>MKYMITSKGDEKSDLLRLNMIAGFGEYDMEYDDVEPEIVISIGGDGTFLS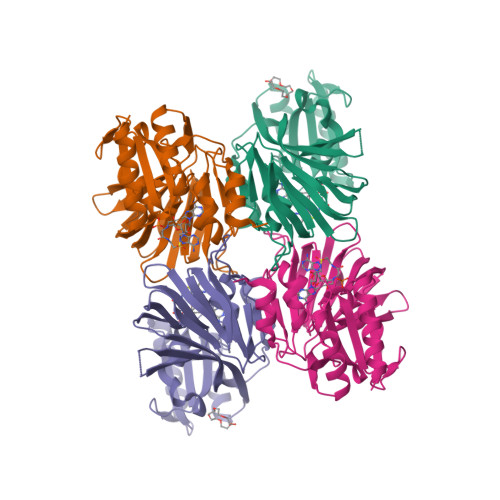AFHQYEERLDEIAFIGIHTGHLGFYADWRPAEADKLVKLLAKGEYQKVSYPLLKTTVKYGIGKKEATYLALNESTVKSSGGPFVVDVVINDIHFERFRGDGLCMSTPSGTTAYNKSLGGALMHPSIEAMQLTEMASINNRVYRTIGSPLVFPKHHVVSLQPVNDKDFQISVDHLSILHRDVQEIRYEVSAKKIHFARFRSFPFWRRVHDSFIEDLEHHHHHH[2x]> GDRVADVIESSIGDSVSRALTQALPAPTGQNTQVSSHRLDTGEVPALQAAEIGASSNTSDESMIETRCVLNSHSTAETTLDSFFSRAGLVGEIDLPLEGTTNPNGYANWDIDITGYAQMRRKVELFTYMRFDAEFTFVACTPTGQVVPQLLQYMFVPPGAPKPESRESLAWQTATNPSVFVKLTDPPAQVSVPFMSPASAYQWFYDGYPTFGEHKQEKDLEYGACPNNMMGTFSVRTVGSSKSKYPLVVRIYMRMKHVRAWIPRPMRNQNYLFKANPNYAGNSIKPTGTSRSAITTL;> SDRVAQLTIGNSTITTQEAANIIVGYGEWPSYCSDDDATAVDKPTRPDVSVNRFYTLDTKLWEKSSKGWYWKFPDVLTETGVFGQNA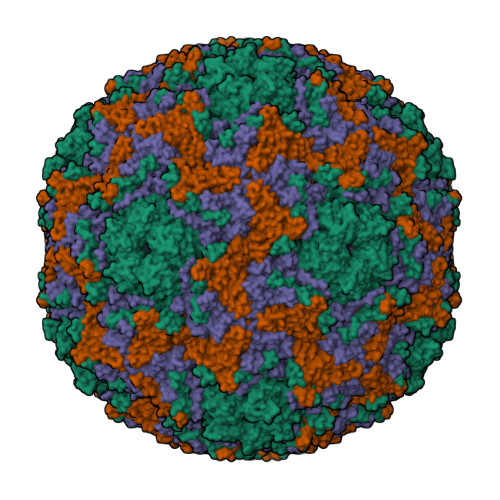QFHYLYRSGFCIHVQCNASKFHQGALLVAILPEYVIGTVAGGTGTEDSHPPYKQTQPGADGFELQHPYVLDAGIPISQLTVCHHQRINLRTNNCATIIVPYMNTLPFDSALNHCNFGLLVVPISPLDFDQGATPVIPITITLAPMCSEFAGLRQAVTQ;> GFPTELKPGTNQFLTTDDGVSAPILPNFHPTPCIHIPGEVRNLLELCQVETILEVNNVPTNATSLMERLRFPVSAQAGKGELCAVFRADPGRDGPWQSTMLGQLCGYYTQWSGSLEVTFMFTGSFMATGKMLIAYTPPGGPLPKDRATAMLGTHVIWDFGLQSSVTLVIPWISNTHYRAHARDGVFDYYTTGLVSIWYQTNYVVPIGAPNTAYIIALAAAQKNFTMKLCKDTSHILQTASIQ;> MGSQVSTQRSGSHENSNSATEGSTINYTTINYYKDSYAATAGKQSLKQDPDKFANPVKDIFTEMAAPLK> GHMQETQAVEAGEKTVEQFVQALNKGDYNKAAEMTSKKAANKSALSEKEILDKYQNIYGAADVKGLQISNLKVDKKDDSTYSFSYKAKMNTSLGELKDLSYKGTLDRNDGQTTINWQPNLVFPEMEGNDKVSLTTQEAARGNIIDRNGEPLATTGKLKQLGVVPSKLGDGGEKTANIKAIASSFDLTEDAINQAISQSWVQPDYFVPLKIIDGATPELPAGATIQEVDGRYYPLGEAAAQLIGYVGDITAEDIDKNPELSSNGKIGRSGLEMAFDKDLRGTTGGKLSITDADGVEKKVLIEHEVQNGKDIKLTIDAKAQKTAFDSLGGKAGSTVATTPKTGDLLALASSPSYDPNKMTNGISQEDYKAYEENPEQPFISRFATGYAPGSTFKMITAAIGLDNGTIDPNEVLTINGLKWQKDSSWGSYQVTAVSDVSQVDLKTALIYSDNIYTAQETLKMGEKKFRTGLDKFIFGEDLDLPISMNPAQISNEDSFNSDILLADTGYGQGELLINPIQQAAMYSVFANNGTLVYPKLIADKETKDKKNVIGETAVQTIVPDLREVVQDVNGTAHSLSALGIPLAAKTGTAEIKEKQDVKG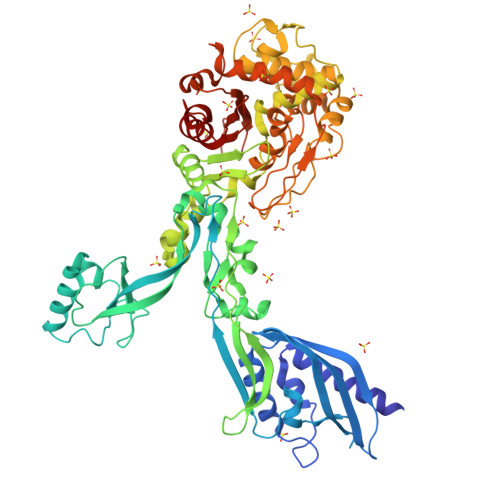KENSFLFAFNPDNQGYMMVSMLENKEDDDSATKRASELLQYLNQNYQ> MSSKYAVKLKTDFDNPRWIKRHKHMFDFLDINGNGKITLDEIVSKASDDICAKLEATPEQTKRHQVCVEAFFRGCGMEYGKEIAFPQFLDGWKQLATSELKKWARNEPTLIREWGDAVFDIFDKD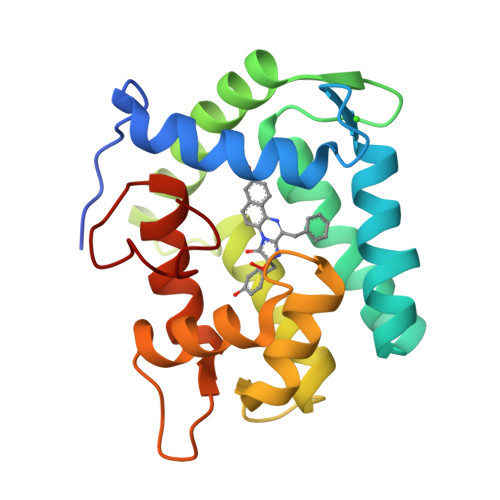GSGTITLDEWKAYGKISGISPSQEDCEATFRHCDLDNAGDLDVDEMTRQHLGFWYTLDPEADGLYGNGVP> IVGGRRARPHAWPFMVSLQLAGGHFCGATLIAPNFVMSAAHCVANVNVRAVRVVLGAHNLSRREPTRQVFAVQRIFEDGYDPVNLLND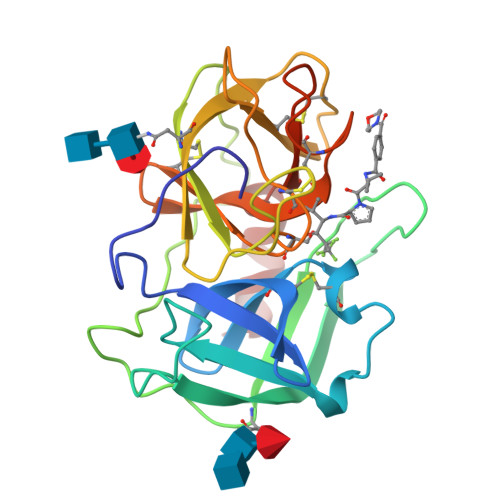IVILQLNGSATINANVQVAQLPAQGRRLGNGVQCLAMGWGLLGRNRGIASVLQELNVTVVTSLCRRSNVCTLVRGRQAGVCFGDSGSPLVCNGLIHGIASFVRGGCASGLYPDAFAPVAQFVNWIDSIIQ>MGLNFFRKAAPEVRTEPVAERKASVTGRIVAMASGAGRPVWGPRDTVSLMRTGFAGNPVGFRSVKLIAEATAAVPLICQDAERRYEIHPVLDLLRRPNAGQGRAELFEALIGQILLSGNGYLEAVCPEPGVPRELHVLRSDRMAVVPGADGWPVGYDYTVGGRKHRFDMTGHPDPICHIKSFHPTDDHYGLSPMQAAAVALDVHNAASAWSKALLDNAARPSGAIIYKGADGQGVLAPEQYERLIFEMETHHQGARNAGRPMLLEGGLDWKPMGFSPSDMEFHETKAAAAREIALAFGVPPMLIGIPGDATYANYAEANRAFYRLTVLPLLTRVSAALAWWLSGYLGAQIELKPDLDQVPALAVERDQLWARIGAAGFLSNSEKRVLLGLPPTAEG[2x];>[11x]MDVFAKHAVSLESPAVRHYEITPSDSTDLARRPRALRVQTGGTLVLRDETGITVTYTVFAGEILPVRPVRVLATGTTATAVGWE;>MPEGADPVAEVKTALAGFLKEVKGFQDDVKTRLQQQEERVTMLQTKTYAGRHALAAAATEEAPHQKAFAAYLRTGDDDGLRGLSLEGKALNSAVAAEGGYLVDPQTSETIRGVLRSTASLRQIASVVNVEATSFDVLVDKTDMGSGWASETAALSETATPQIDRITIPLHELAAMPKASQRLLDDSAFDIETWLANRIADKFARAEAAAFISGDGVDKPTGFLTKTKVANGAWAWGSLGYVATGAAGDFAAVNASDAVVDLVYALGAEYRANASFVMNSKTAGAVRKMKDADGRFLWADSLAAGEPARLMGYPVLIAEDMPDIAANAYAIAFGDFGNGYTIAERPDLRVLRDPFSAKPHVLFYASKRVGGDVSDFAAIKLLKFAA[29x];>[2x]MMLNEVTAVPGTALPVAEFRDHLRLGTGFADLGAEDAALLSYLRAAIAAIEGRTAKALISRGFRLALTAWRWGDMQTLPIAPVATVTALRLVDAAGVETPVAAGWRLVPDMARPRIEALGAMLPMIPTGGRVEIDFTAGFGASWSALPVDLAQAVFLLAAQYYELRHDGAAEGGAMPFGVMALIERWRTVRVLGGRP;> MSRPRLNRLLVLEEAVRVADGAGGHRLDWQAKGEVWAEVTAGSGSERAGEFVTLASVPFTIVVRAAPVGAARRPRPEQRFREGARIFRILAVAERDREGHYLSCFAREEVVA;> MSYAVAGALQAAVYQQLRADAVLAALVGTAVYDAVPPGPLAGTYVSLGPEDVADASDKTGAGAVHDFVISVITDAAGFATAKAAAAAVSDALVGADLVLSRGRLVGLWFLRAKARRVEKADMRRIDLVFRARVEG;>MIALGLGLGLAANGGPALRRYAVNGVAPVAVLDFERHFLSHPLALTRATSATYADALRAVQTAPADTPRYDYSTGKRALLLEASATNLLPNSAQFEAASWGKTRASVLANAALAPNGTMTADKLVEDTSNNSHFVARTGTQIAAGTSVTASIFVKAAERRWFALVTADSANAFRTTYFDLQTGTLGVVSQGAAGHVAQIVAAGNGWYRCSVTQTQAASGNFNFYPSVASANGATSYPGDGASGLYLWGAQLEAGAAVSSVIPTEAAAVTRAADLASVAVAAGSYDLRRVDAAGTAVTKGVAHPGGALTIGAGSLYLLSLFPAGAL[2x];>MAAQNGKDLLIKLDLTGSGQFETIAGLRATRISFNAETVDVTSLESQGGWRELLGGAGVRSASISGAGVFKDADTDERARQIFFDGEVPEFQVIIPDFGIVQGPFMITSIDYAGSHNGEASYELAMASAGALSFTAI[4x]

Gene transfer agents (GTAs) are DNA-containing phage-like particles produced by some species of bacteria and archaea. The genes encoding proteins that form Rhodobacter capsulatus GTA particles (RcGTA) are derived from phage DNA, which has been integrated into the bacterial genome. Here, we use cryo-electron microscopy (cryo-EM) to determine the structures of RcGTA before and after DNA ejection, and to visualize the interactions of RcGTA with R. capsulatus cells. Particles of RcGTA have heads with a diameter of 38-nm and 49-nm long tails.

The iris has to open to enable genome ejection. Therefore, the release of DNA from the RcGTA particle requires re-arrangement of the baseplate, which is consistent with the observation that one third of empty RcGTA particles lacked baseplates. The central channel of the RcGTA tail above the iris contains a trimer of tape measure proteins and perhaps also one molecule of peptidoglycan peptidase. These proteins have to be released from the virion before the DNA can exit. Some of the empty particles with the baseplate still present contained density corresponding to the inner tail proteins, which would not allow the DNA ejection through the tail. We speculate that the empty particles with attached baseplate are defective and never contained a full complement of DNA. The structure of tail tube did not reveal any changes after DNA ejection, suggesting that the tail is not involved in signaling to trigger DNA ejection after attachment to a cell.(3aR,4R,6R,7R,8aR)-6-phenyloctahydro-1H-3a,7-epiminocyclohepta[c]pyrrol-4-ol | C15 H20 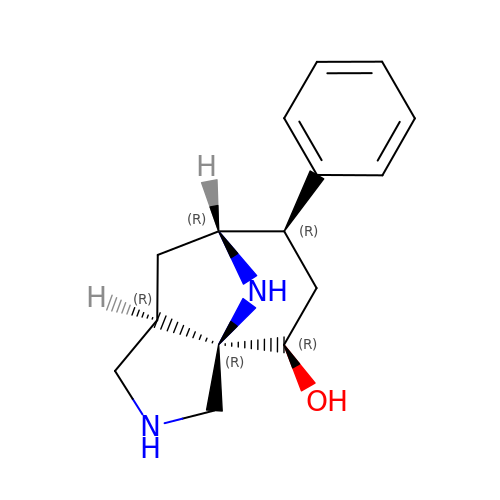N2 O | WNBPFOXFPIFLPO-RYPNDVFKSA-N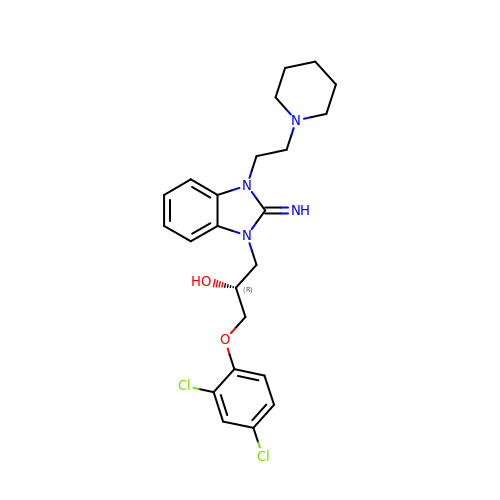(2R)-1-(2,4-dichlorophenoxy)-3-[(2E)-2-imino-3-(2-piperidin-1-ylethyl)-2,3-dihydro-1H-benzimidazol-1-yl]propan-2-ol | C23 H28 Cl2 N4 O2 | QMRFKZWWZBZQKJ-MVXIZWJUSA-N>AAGAAPVDISTLPRVKVDLVKPPFVHAHDQVAKTGPRVVEFTMTIEEKKLVIDREGTEIHAMTFNGSVPGPLMVVHENDYVELRLINPDTNTLLHNIDFHAATGALGGGALTQVNPGEETTLRFKATKPGVFVYHCAPEGMVPWHVTSGMNGAIMVLPRDGLKDEKGQPLTYDKIYYVGEQDFYVPKDEAGNYKKYETPGEAYEDAVKAMRTLTPTHIVFNGAVGALTGDHALTAAVGERVLVVHSQANRDTRPHLIGGHGDYVWATGKFRNPPDLDQETWLIPGGTAGAAFYTFRQPG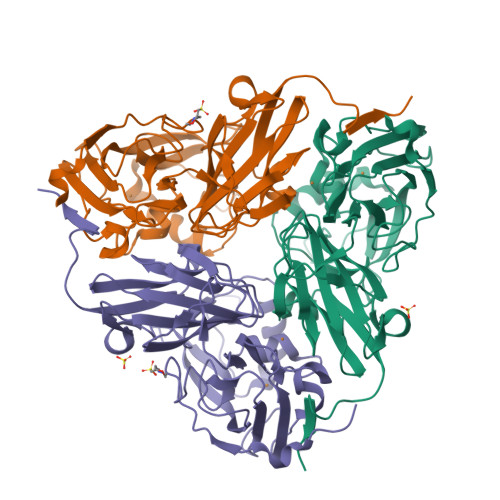VYAYVNHNLIEAFELGAAGHFKVTGEWNDDLMTSVV[3x]> MSDKKTQTRARILGAATQALLERGAVEPSVGEVMGAAGLTVGGFYAHFQSKDALMLEAFEQLLGKRRELLGELDPGLSGKERRALAAAFYLSRKHRDAQVDAGCPLPATLAEVARLPEGFREVLSRHVEIMVTSLAESPEETDVALADLVL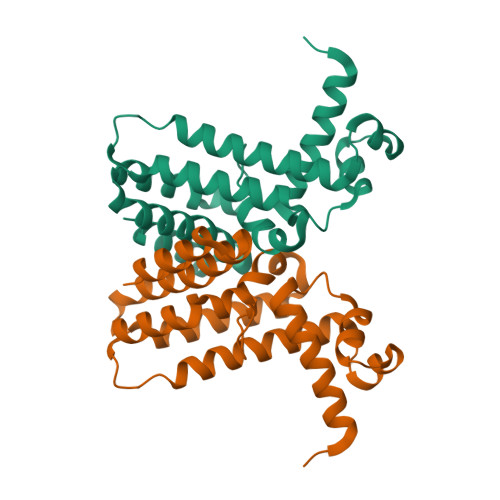MIGGLALARALGPGELSDRVLRAAKQAVN>MEKQQDLPFPYEFRELNPEEDKLVKANLGAFPTTYVKLGPKGYMVYRPYLKDAANIYNMPLRPTDVFVASYQRSGTTMTQELVWLIENDLNFEAAKTYMSLRYIYLDGFMIYDPEKQEEYNDILPNPEN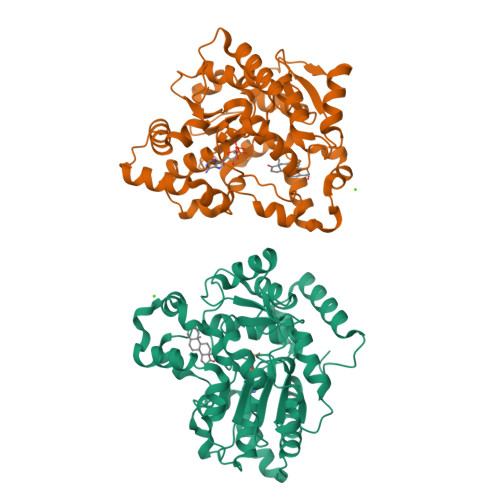LDMERYLGLLEYSSRPGSSLLAAVPPTEKRFVKTHLPLSLMPPNMLDTVKMVYLARDPRDVAVSSFHHARLLYLLNKQSNFKDFWEMFHRGLYTLTPYFEHVKEAWAKRHDPNMLFLFYEDYLKDLPGSIARIADFLGKKLSEEQIQRLSEHLNFEKFKNNGAVNMEDYREIGILADGEHFIRKGKAGCWRDYFDEEMTKQAEKWIKDNLKDTDLRYPNMEL[2x]> APVAAYVDEVLNEVLVVPNINQSHPTTSNAAPVLDAAETGHTNKIQPEDTIETRYVQSSQTLDEMSVESFLGRSGCIHESVLDIVDNYNDQSFTKWNINLQEMAQIRRKFEMFTYARFDSEITMVPSVAAKDGHIGHIVMQYMYVPPGAPIPTTRDDYAWQSGTNASVFWQHGQPFPRFSLPFLSIASAYYMFYDGYDGDTYKSRYGTVVTNDMGTLCSRIVTSEQLHKVKVVTRIYHKAKHTKAWCPRPPRAVQYSHTHTTNYKLSSEVHNDVAIRPRTNLTTV;> SDRIIQITRGDSTITSQDVANAVVGYGVWPHYLTPQDATAIDKPTQPDTSSNRFYTLDSKMWNSTSKGWWWKLPDALKDMGIFGENMFYHFLGRSGYTVHVQCNASKFHQGTLLVVMIPEHQLATVNKGNVNAGYKYTHPGEAGREVGTAAAAEKQPSDDNWLNFDGTLLGNLLIFPHQFINLRSNNSATLIVPYVNAVPMDSMVRHNNWSLVIIPVCQLQSNNISNIVPITVSISPMCAEFSGARAKTVVQ;> GLPVYVTPGSGQFMTTDDMQSPCALPWYHPTKEIFIPGEVKNLIEMCQVDTLIPINSTQSNIGNVSMYTVTLSPQTKLAEEIFAIKVDIASHPLATTLIGEIASYFTHWTGSLRFSFMFCGTANTTLKVLLAYTPPGIGKPRSRKEAMLGTHVVWDVGLQSTVSLVVPWISASQYRFT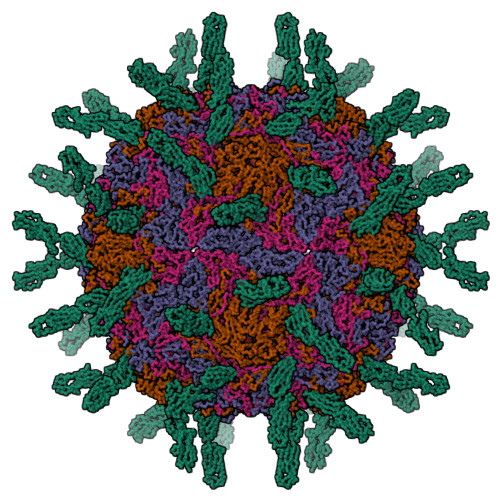TPDTYSSAGYITCWYQTNFVVPPNTPNTAEMLCFVSGCKDFCLRMARDTDLHKQTGPITQ;> GAQVSRQNVGTHSTQNMVSNGSSLNYFNINYFKDAASSGASRLDFSQDPSKFTDPVKDVLEKGIPTLQ;> QTSVSPSKVILPRGGSVLVTCSTSCDQPKLLGIETPLPKKELLLPGNNRKVYELSNVQEDSQPMCYSNCPDGQSTAKTFLTVYWTPERVELAPLPSWQPVGKNLTLRCQVEGGAPRANLTVVLLRGEKELKREPAVGEPAEVTTTVLVRRDHHGANFSCRTELDLRPQGLELFENTSAPYQLQTF structures of the Mep2 transceptors from S. cerevisiae and C. albicans. function as ammonium receptors/sensors in fungal development. a central channel for the transport of ammonium. non-phosphorylated, with channels that are closed on the cytoplasmic side.

The Mep2 protein of S. cerevisiae (ScMep2) was overexpressed in S. replacement (MR) with the archaebacterial Amt-1 structure (see Methods section). the otherwise highly similar Mep2 proteins of S. cerevisiae and C. within the N terminus, intracellular loops (ICLs) ICL1 and ICL3, and the CTR. extracellular loop ECL5 of a neighbouring monomer.

>[9x]MSYNFTGTPTGEGTGGNSLTTDLNTQFDLANMGWIGVASAGVWIMVPGIGLLYSGLSRKKHALSLLWASMMASAVCIFQWFFWGYSLAFSHNTRGNGFIGTLEFFGFRNVLGAPSSVSSLPDILFAVYQGMFAAVTGALMLGGACERARLFPMMVFLFLWMTIVYCPIACWVWNAEGWLVKLGSLDYAGGLCVHLTSGHGGLVYALILGKRNDPVTRKGMPKYKPHSVTSVVLGTVFLWFGWMFFNGGSAGNATIRAWYSIMSTNLAAACGGLTWMVIDYFRCGRKWTTVGLCSGIIAGLVGITPAAGFVPIWSAVVIGVVTGAGCNLAVDLKSLLRIDDGLDCYSIHGVGGCIGSVLTGIFAADYVNATAGSYISPIDGGWINHHYKQVGYQLAGICAALAWTVTVTSILLLTMNAIPFLKLRLSADEEELGTDAAQIGEFTYEESTAYIPEPIRSKTSAQMPPPHENIDDKIVGNTDAEKNSTPSDASSTKNTDHIVHHHHHH> NTKYNKEFLLYLAGFVDSDGSIIAQIKPNQSVKFKHRLQLTFDVTQKTQRRWFLDKLVDEIGVGYVADSGSVSKYRLSEIKPL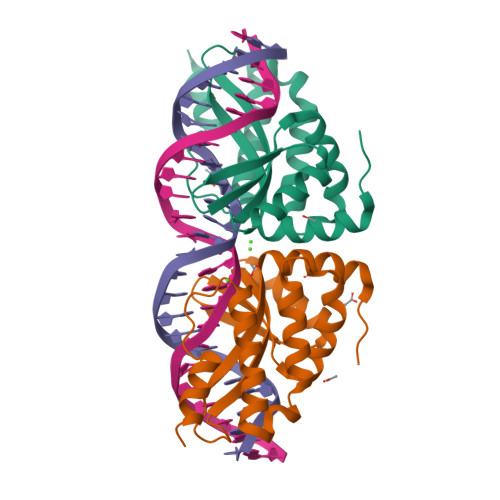HNFLTQLQPFLKLKQKQANLVLKIIEQLPSAKESPDKFLEVCTWVDQIAALNDSKTRKTTSETVRAVLDS;> NTKYNKEFLLYLAGFVDGDGSIIAQIKPNQSGKFKHKLSLTFKVTQKTQRRWFLDKLVDEIGVGYVYDSGSVSNYYLSEIKPLHNFLTQLQPFLKLKQKQANLVLKIIEQLPSAKESPDKFLEVCTWVDQVAALNDSKTRKTTSETVRAVLDSL>MSPRSRLLASSLRGGLLLRPCSARRSTLLNPSPSPLRKAIFHTTSLRAFKNLAEIATSSKEDASSLKPKGKPSPPGDPLATIEKTAAEQRRADWAIIKQMSRYLWPKDSWSDKARVLLALSLLVGGKVLNVHVPFYFREIIDRLNIDVAAVGGTVSAVAGAVIFAYGASRIGAVVSQELRNAVFSSVAQKAIRRVATQTFGHLLNLDLSFHLSKQTGGLTRAIDRGTKGISYLLTSMVFHIVPTALEIGMVCGILTYQFGWEFAAITAATMAAYTAFTITTTAWRTKFRRQANAADNAASTVAVDSLINYEAVKYFNNEAYEIARYDKALQAYERSSIKVATSLAFLNSGQNIIFSSALTLMMWLGARGVLAGDLSVGDLVLINQLVFQLSVPLNFLGSVYRELRQSLLDMETLFDLQKVNVTIREAPNAKPLALPKGGEIRFENVTFGYYPDRPILRNLSLTIPAGKKVAVVGPSGCGKSTLL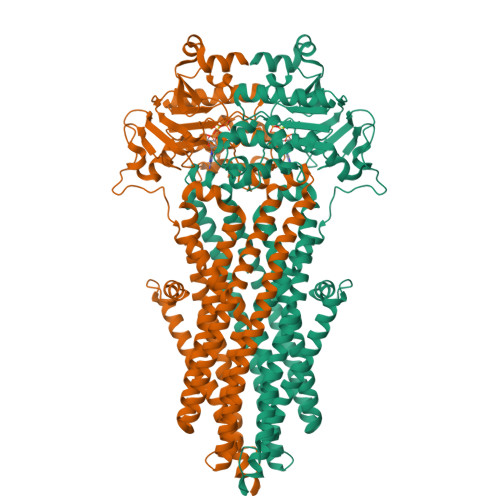RLLFRSYDPQQGKIFIDDQDIKSVTLESLRKSIGVVPQDTPLFNDTVELNIRYGNVNATQEQVIAAAQKAHIHEKIISWPHGYQTRVGERGLMISGGEKQRLAVSRLILKDPPLLFFDQATSALDTHTEQALMANINEVVKEKKRTALFVAHRLRTIYDADLIIVLKEGVVVEQGSHRELMERDGVYAELWMAQEMLHQGEAAEEPAEGEKAEEKK[2x]>[2x]MSSRKELANAIRALSMDAVQKAKSGHPGAPMGMADIAEVLWRDFLKHNPQNPSWADRDRFVLSNGHGSMLIYSLLHLTGYDLPMEELKNFRQLHSKTPGHPEVGYTAGVETTTGPLGQGIANAVGMAIAEKTLAAQFNRPGHDIVDHYTYAFMGDGCMMEGISHEVCSLAGTLKLGKLIAFYDDNGISIDGHVEGWFTDDTAMRFEAYGWHVIRDIDGHDAASIKRAVEEARAVTDKPSLLMCKTIIGFGSPNKAGTHDSHGAPLGDAEIALTREQLGWKYAPFEIPSEIYAQWDAKEAGQAKESAWNEKFAAYAKAYPQEAAEFTRRMKGEMPSDFDAKAKEFIAKLQANPAKIASRKASQNAIEAFGPLLPEFLGGSADLAPSNLTLWSGSKAINEDAAGNYIHYGVREFGMTAIANGISLHGGFLPYTSTFLMFVEYARNAVRMAALMKQRQVMVYTHDSIGLGED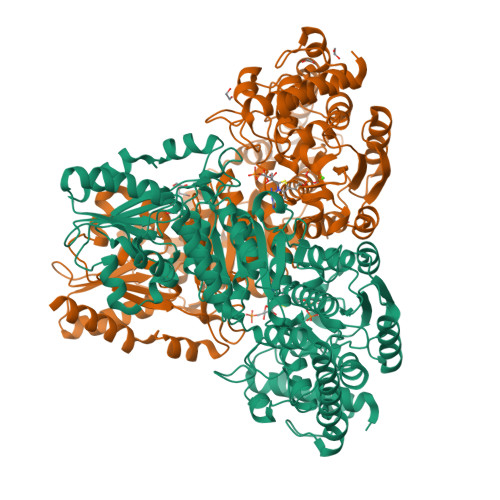GPTHQPVEQVASLRVTPNMSTWRPCDQVESAVAWKYGVERQDGPTALILSRQNLAQQERTEEQLANIARGGYVLKDCAGQPELIFIATGSEVELAVAAYEKLTAEGVKARVVSMPSTDAFDKQDAAYRESVLPKAVTARVAVEAGIADYWYKYVGLNGAIVGMTTFGESAPAELLFEEFGFTVDNVVAKAKELLHHHHHH>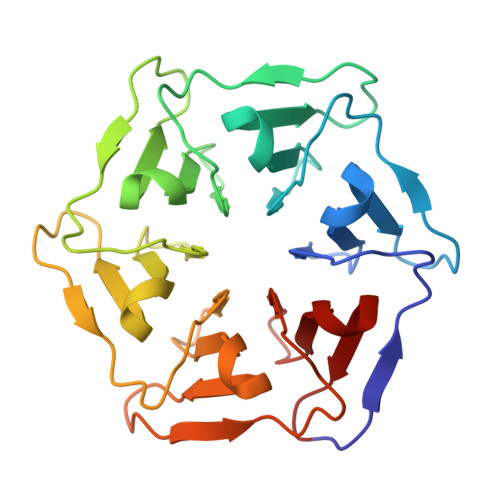SNTQTVLPFTGLNTPSGVAVDSAGTVWVTDHGNNRVVKLAAGSNTQTVLPFTGLNTPSGVAVDSAGTVWVTDHGNNRVVKLAAGSNTQTVLPFTGLNTPSGVAVDSAGTVWVTDHGNNRVVKLAAGSNTQTVLPFTGLNTPSGVAVDSAGTVWVTDHGNNRVVKLAAGSNTQTVLPFTGLNTPSGVAVDSAGTVWVTDHGNNRVVKLAAGSNTQTVLPFTGLNTPSGVAVDSAGTVWVTDHGNNRVVKLAAG[2x]>[4x]MSLRHLYIEEGRTVCASATSRNRRPTSESPHSDDVVVVEGML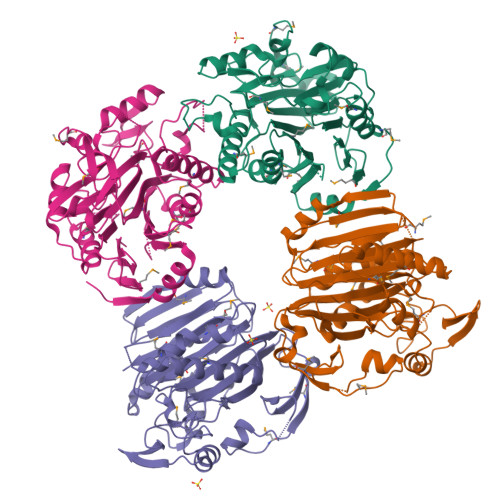RGRPETRVHAMFDGFQGRHSAMWLAQNVMNYLNDLRDVNEEEITRQFERMDGDLRAANLPGGSSALIIFVRYEKKPTEARVVGRQIVPEGAKEFTSVAEALGGPLMPVVAMNFRRDPRAAKGIYTIHVASLGNSRCVLKSGRTAIHLSTPHTASSHKERHRVQAAGGVFTTVNGELLLGGVVPMTRAFGSFDFKKGGQGKLQQDLVSAVPDVTTFFAYPGDDIVAGTAGAFAHFRSHAAIAAAIALYPVSPETVLDAAKAMVVNAKRRKVTKNISTFVRHLPESRTRSQKMLEGTSGENGEEDFSIDRTNELTQALQAGFFSFLLYYEGHHHHHH> VRSSSRTPSDKPVAHVVANPQAEGQLQWLNRRANALLANGVELRDNQLVVPSEGLYLIYSQVLFKGQGCPSTHVLLTHTISRIAVSYQTKVNLLSAIKSPCQRETPEGAEAKPWYEPIYLGG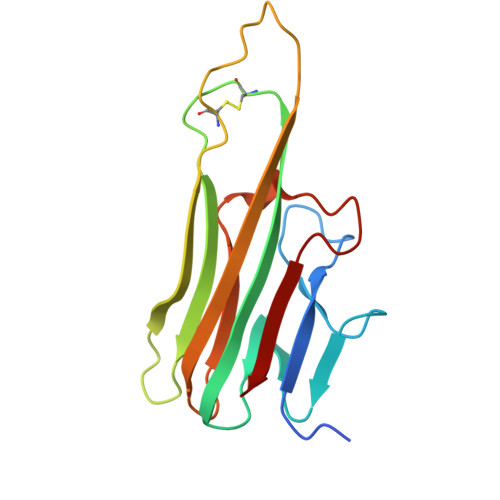VFQLEKGDRLSAEINRPDYLDFAESGQVYFGIIAL>[2x]MDLKPDWVVGFVDGEGCFYVGVSRNRTMKTGYQVLPEFRIVQHKRDIQVLYALRKFFGCGVVRKNHDDRYELRIRKRSCLKKVVEFFEKHPLKTKKNVDFKKFRRILIMMERGEHLTKEGLI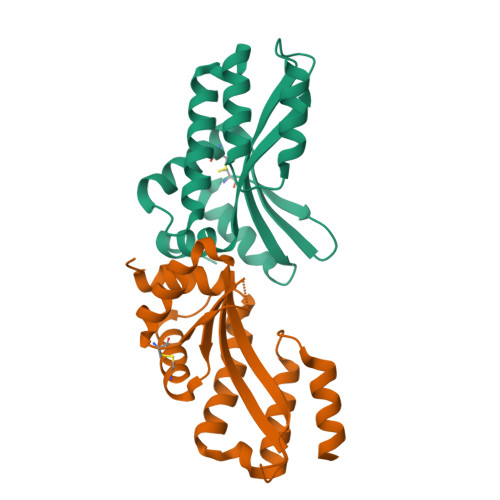KILEIAMEMNTGNHERLKRTLEEIRGLDEDTVHPHSERVGLEHHHHHH>MAATRDVTHLTDISKGLAEADGSFKRKASTFRRFIEKGGEFEPEKGRYHLYVAYSSPWATRT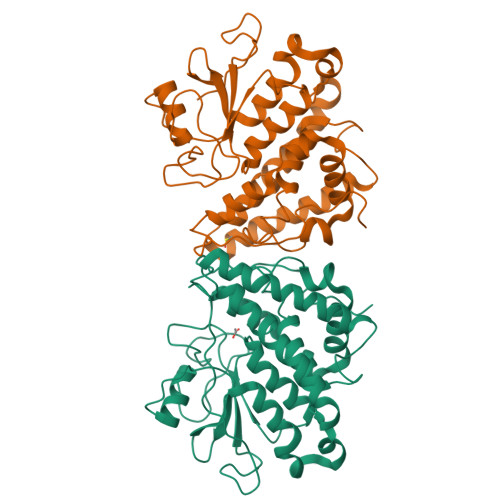LIVRKIKGLEEIVGVTIVSPLFSAHGWPFGDVSPFPGAEADPFYNAQYVRDLYLRADPKYEGRFTVPVLWDKKTETVVNNESSEIIRIFNTAFNEFLPADKAAIHLYPEALKSEIDEINEWVYDTVNNGVYKAGFATTQQAYEAAVIPLFESLDRLEKILTGKDYLVGDQLTEADVRLFVTIIRFDPAYVGHFKCNLRTIRDGYPAIHLWLRKLYWNNSAFSETCKFDHIKASYYAQKNVNPTLVVPLGPIPNILPLHHHHHH[2x]> GVSGFQRLQKPVVSQPDFRRQPVSETMQVYLKQAADPGRDVGLYWMATDFENRRFPGKVSPSGFQKLYRQWRNQTGWDAYVQSCRAIWNDVKYFPIPQSLDDTEDKISYVDSWMFERNYGGKRGHEGTDIMAEKNTPGYYPVVSMTDGVVTEKGWLEKGGWRIGITAPTGAYFYYAHLDSYAELEKGDPVKAGDLLGYMGDSGYGEEGTTGEFPVHL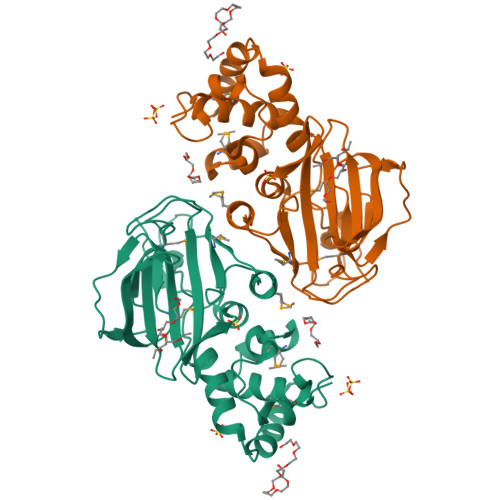HLGIYLKEGTEEISVNPYPVLRYAENARIKCVYSR>MHNLQQLLPTRSLIWIFSFLTSISIWCTVAHAETEGRVQHFTGYIEDGRGIFYSLPDMKQGDIIYASMQNTGGNLDPLVGIMAEEIDPAVSLGQVLEKALASENDLISELTAVADRIFLGWDDDGGKGYSASLEFTIPRDGTYHIFAGSTITNQRLDKFQPTYTTGSFQLILGLNAPQVISGEGEPEGEVFASLASLEIKPEAHVQELEIRLDKDTRYLTQHTRNLQPGDTFHALVEPIGEAPLPRLRLTDSGGKPLAFGLIDQPGESVELNYTCDQDICELVVHVDGTDGQKDSGEAVYRLLVGINAPNLRESGQTPVGSSVFLESDLVTVGLAVDQIVGVDQRSENFSVVGTLKLSWHDPKLGFSPDQCGCTVKSFEDASIRAVAGEINLPLPSFSFYNQQGNRWSQNQVIFVTPDGRASYFERFTVTLQAPDFDFLAYPFDRQKFSIKVDLAVPTNMFIFNEIERFQQVVGDQLGEEEWVVTSYSQEITEVPFERGSTNSRFTTTLLVKRNLEYYILRIFVPLFLIISVSWVIFFL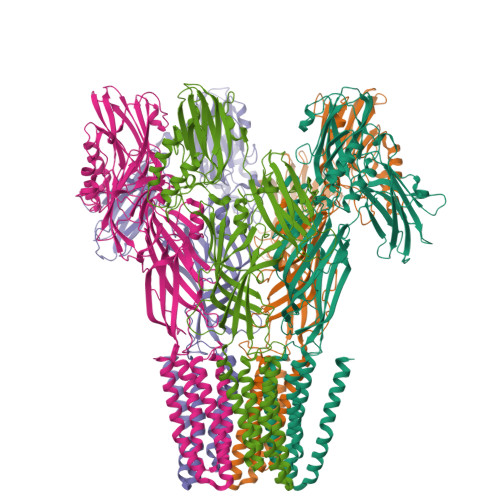KDYGRQLEVASGNLLVFVAFNFTISGDLPRLGYLTVLDRFMIVSFCLTAIVVLISVCQKRLGAVGKQAVAAQIDTWVLVIYPLVYSLYIIWVYLRFFTDHIGW[5x]>[6x]MRKFRLIPYKQVDKVSALSEVPMGVEIVEAPAVWRASAKGAGQIIGVIDTGCQVDHPDLAERIIGGVNLTTDYGGDETNFSDNNGHGTHVAGTVAAAETGSGVVGVAPKAD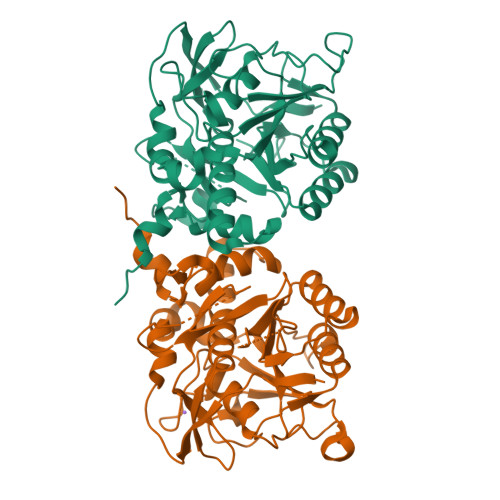LFIIKALSGDGSGEMGWIAKAIRYAVDWRGPKGEQMRIITMSLGGPTDSEELHDAVKYAVSNNVSVVCAAGNEGDGREDTNEFAYPAAYNEVIAVGAVDFDLRLSDFTNTNEEIDIVAPGVGIKSTYLDSGYAELSGTAMAAPHVAGALALIINLAEDAFKRSLSETEIYAQLVRRATPIGFTAQAEGNGFLTLDLVERITGQFTEKGKKLEHHHHHH The most well-studied baculovirus is Autographa californica multiple nucleopolyhedrovirus (AcMNPV). Baculoviruses have their large circular dsDNA genome packaged into an enveloped rod-shaped nucleocapsid. The BV nucleocapsid structure consists of three parts, a central helical sheath containing the viral genome, an apical cap and a basal structure attached to both extremities of the helical sheath. Herein, we report high-resolution cryo-electron microscopy (cryo-EM) structures of the BV nucleocapsid combined with de novo modeling and Alphafold predictions.

The outer rings of the basal structure and the apical cap follow a C14 symmetry and connect the cap complexes with the helical portion of the nucleocapsid, functioning as an anchor. We term this structure the ‘anchor’ complex. It is organized in a two-ring structure, referred to here as anchor-1 for its most peripheral part and anchor-2 for the inner one (Fig. 1 and Supplementary Fig. 4D–G (basal), Supplementary Fig. 9E, F (apical)). On the similarity, common proteins for both basal and apical anchor complexes include Ac142, Ac109, Ac104, VP39 for anchor-1 and Ac101 (also known as C42 or P40) and Ac144 (E27) for anchor-211. Notably, the arrangement of three Ac104 molecules and their interactions with VP39, Ac109 and Ac142 in the apical anchor-1 ring mirrors the equivalent basal arrangement observed in both our BV structures and the recently reported ODV structure. A major difference between the anchor-2 complexes in the apical and basal structures is the presence of Ac98 in the basal anchor-2, which interacts exclusively with Ac144 from the lowermost Ac101/Ac144 module. Nevertheless, this interaction with Ac98 has very little consequence on the structure of Ac144 or on the rest of the anchor-2. For both the apical and basal ends, the nucleocapsid’s elongated tubular section, composed of helically organized VP39 dimers, terminates with Ac109 binding. Additionally, the VP39 lattice transitions from a straight to a curved shape due to interaction with proteins forming the anchor-1 and −2 rings. The main influencing factor for the curvature is the presence of three Ac104 copies per asymmetric unit, each interacting with a distinct VP39 monomer.

>[2x]MKRIKCNKVRTVTEIVNSDEKIQKTYELAEFDLKNLSSLESYETLKIKLALSKYMAMLSTLEMTQPLLEIFRNKADTRQIAAVVFSTLAFIHNRFHPLVTNFTNKMEFVVTETNDTSIPGEPILFTENEGVLLCSVDRPSIVKMLSREFDTEALVNFENDNCNVRIAKTFGASKRKNTTRSDDYESNKQPNYDMDLSDFSITEVEATQYLTLLLTVEHAYLHYYIFKNYGVFEYCKSLTDHSLFTNKLRSTMSTKTSNLLLSKFKFTIEDFDKINSNSVTSGFNIYNFNK;>MSAIALYLEINKLRLKIDEPMQLAIWPQLFPLLCDEHQSVQLNTDVLINFMMHVARKSQNTILNNNAAIASQYAAGNADVVAAPASAQPTPRPVINLFARANAAAPAQPSEELINMRRYRNAARKLIHHYSLNSTSSTEYKISDVVMTMIFLLRSEKYHSLFKLLETTFDDYTCRPQMTQVQTDTLLDAVRSLLEMPSTTIDLTTVDIMRSSFARCFNSPIMRYAKIVLLQNVALQRDKRTTLEELLIERGEKIQMLQPQQYINSGTEIPFCDDAEFLNRLLKHIDPYPLSRMYYNAANTMFYTTMENYAVSNCKFNIEDYNNIFKVMENIRKHSNKNSNDQDELNIYLGVQSSNAKRKKY[2x];> MASSLQSKWICLRLNDAIIKRHVLVLSEYADLKYLGFEKYKFFEYVIFQFCNDPQLCKIIENNYNYCMQIFKAPADDMRDIRHNIKRAFKTPVLGHMCVLSNKPPMYSFLKEWFLLPHYKVVSLKSESLTWGFPHVVVFDLDSTLITEEEQVEIRDPFVYDSLQELHEMGCVLVLWSYGSRDHVAHSMRDVDLEGYFDIIISEGSTVQEERSDLVQNSHNAIVDYNLKKRFIENKFVFDIHNHRSDNNIPKSPKIVIKYLSDKNVNFFKSITLVDDLPTNNYAYDFYVKVKRCPTPVQDWEHYHNEIIQNIMDYEQYFIK;> MSGGGNLLTLERDHFKYLFLTSYFDLKDNEHVPSEPMAFIRNYLNCTFDLLDDAVLMNYFNYLQSMQLKHLVGSTSTNIFKFVKPQFRFVCDRTTVDILEFDTRMYIKPGTPVYATNLFTSNPRKMMAFLYAEFGKVFKNKIFVNINNYGCVLAGSAGFLFDDAYVDWNGVRMCAAPRLDNNMHPFRLYLLGEDMAKHFVDNNILPPHPSNAKTRKINNSMFMLKNFYKGLPLFKSKYTVVNSTKIVTRKPNDIFNEIDKELNGNCPFIKFIQRDYIFDAQFPPDLLDLLNEYMTKSSIMKIITKFVIEENPAMSGEMSREIILDRYSVDNYRKLYIKMEITNQFPVMYDHESSYIFVSKDFLQLKGTMNAFYAPKQRILSILAVNRLFGATETIDFHPNLLVYRQSSPPVRLTGDVYVVDKNEKVFLVKHVFSNTVPAYLLIRGDYESSSDLKSLRDLNPWVQNTLLKLLIPDSVQ;>MALVPVGMAPRQMRVNRCIFASIVSFDACITYKSPCSPDAYHDDGWFICNNHLIKRFKMSKMVLPIFDEDDNQFKMTIARHLVGNKERGIKRILIPSATNYQDVFNLNSMMQAEQLIFHLIYNNENAVNTICDNLKYTEGFTSNTQRVIHSVYATTKSILDTTNPNTFCSRVSRDELRFFDVTNARALRGGAGDQLFNNYSGFLQNLIRRAVAPEYLQIDTEELRFRNCATCIIDETGLVASVPDGPELYNPIRSSDIMRSQPNRLQIRNVLKFEGDTRELDRTLSGYEEYPTYVPLFLGYQIINSENNFLRNDFIPRANPNATLGGGAVAGPAPGVAGEAGGGIAV[4x];>MNDSNSLLITRLAAQILSRNMQTVDVIVDDKTLSLEEKIDTLTSMVLAVNSPPQSPPRVTSSDLAASIIKNNSKMVGNDFEMRYNVLRMAVVFVKHYPKYYNETTAGLVAEIESNLLQYQNYVNQGNYQNIEGYDSLLNKAEECYVKIDRLFKESIKKIMDDTEAFEREQEAERLRAEQTAANALLERRAQTSADDVVNRADANIPTAFSDPLPGPSAPRYMYESSESDTYMETARRTAEHYTDQDKDYNAAYTADEYNSLVKTVLLRLIEKALATLKNRLHITTIDQLKKFRDYLNSDADAGEFQIFLNQEDCVILKNLSNLASKFFNVRCVADTLEVMLEALRNNIELVQPESDAVRRIVIKMTQEIKDSSTPLYNIAMYKSDYDAIKNKNIKTLFDLYNDRLPINFLDTSATSPVRKTSGKRSAEDDLLPTRSSKRANRPEINVISSEDEQEDDDVEDVDYEKESKRRKLEDEDFLKLKALEFSKDIVNEKLQKIIVVTDGMKRLYEYCNCKNSLETLPSAANYGSLLKRLNLYNLDHIEMNVNFYELLFPLTLYNDNDNSDKTLSHQLVNYIFLASNYFQNCAKNFNYMRETFNVFGPFKQIDFMVMFVIKFNFLCDMRNFAKLIDELVPNKQPNMRIHSVLVMRDKIVKLAFSNLQFQTFSKKDKSRNTKHLQRLIMLMNANYNVI[3x];> MECPFQIQVCISDRFFAFPHNLVEPQSDVGNKLIENLIVYVPTDDDRLYIDKKQFPKFNSVLVYRHEHDVNIDSRSPKKTASATIVYWNPLVPITEIGAGETRVFSVLLTNNLFYCNTMIVHHENPKCPIEFTYPETDMQSACSALLKNRNGQSVPPPIKSNLRPIACEIPLSHFKELVESNDFLLCFNLETSTMVKILSLKRIFCIFQYRKQPARYVINLPHEEIDNLYNKLNWERTRRLMKGDVPSNCATVNRSSLKYIKQAQSLLGIPDYSQTVVDFVKMFQKIIFPYQLVPNVIIKLNNFDQMVSSAPNKAEPYKKIRLFCKNDSIAISSSGIVPINMPDFSPPNTFDYSDYANRTNINFVTQRVLTDGGFSSGITVTPVKYNYYL>[2x]MLSNLKTGNNILGLPEFELNGCRFLYKKGIEKTIITFSAFPPKDIAQKYNYIKDFLSSNYTFLAFLDTKYPEDDARGTYYITNELDNGYLQTIHCIIQLLSNTNQEDTYLLGSSKGGVGALLLGLTYNYPNIIINAPQAKLADYIKTRSKTILSYMLGTSKRFQDINYDYINDFLLSKIKTCDSSLKWNIHITCGKDDSYHLNELEILKNEFNIKAITIKTKLISGGADNEAIAHYREYFKTIIQNILEHHHHHH

The key enzyme is the O-acetyltransferase CsaC (MynC) encoded in region A of the CPS gene cluster. Our structural analysis of CsaC identified the capsule O-acetyltransferase of NmA as an α/β-fold enzyme with Ser-His-Asp triad. Each protomer consists of a central eight-stranded β-sheet that is sandwiched by six α-helices and capped by a lid area formed by helices α5, α6, and α7. A deep positively charged groove, which traverses the protein surface, allows substrate binding and opens into an active site that is characterized by a catalytic triad composed of S114, H228 and D198.

As soaking of CsaC-WT crystals with acetyl-CoA or CoA yielded only incomplete substrate density and co-crystallization trials were unsuccessful, we soaked crystals of the catalytically impaired variant H228A with acetyl-CoA. All protomers showed complete density for CoA with a free SH-group. Concomitantly, the triad serine showed an extended electron density with a contour indicative of its O-acetylated form (AcS114). This suggests that CsaC adopted the double displacement mechanism of ABH esterases and forms a transient acetyl-enzyme intermediate that is trapped in the absence of H228. CoA, as the first reaction product, is bound along the positively charged groove in an L-shaped conformation. The pantetheine moiety is engaged in hydrophobic contacts (I233, A39, and F40), and only the distal carbonyl oxygen is specifically recognized by S113-Oγ, a contact that directs the SH-group towards the triad serine S114. The purine nucleobase of CoA is sandwiched between I11 and K48 and locked into position by a hydrogen bond between adenine-N7 and Y49-N, while the phosphate oxygens of the ADP-3′-phosphate moiety are encased by a hydrogen network provided by R237, K53, Y51 and I52. In the H228A(-AcS114)-CoA complex, Q138 positions AcS114, which is approached on the opposite side by the SH-group of CoA. CsaC-H228A, in contrast, showed no detectable adduct hydrolysis, demonstrating an essential function of H228 in the second half-reaction, i.e., transfer of the acetyl group from AcS114 to the acceptor (CPS or water). In support of our hypothesis that Q138 can substitute H228 as a general base in the first half-reaction, Q138 is optimally positioned in both CsaC-WT and the CsaC-H228A(-AcS114)-CoA complex and impaired acetyl-adduct formation was seen upon simultaneous replacement of H228 and Q138.>HHHHHHSSGLVPRGSHMQTTTVYSLEDLLPYLKQDNVDVKLAPGTYNVNGFDVGEDRLFSTTPLFLFEGSNSTYDFTDVKLNINTVVLTKFGNNEVNEIQILGNNNVLKNLKLEDIGTTAPSNRAQSIVIDGRDNRIEGFHLTIRGSYPYGYGDAFGKGGGSVINHRKHSGVLIRGLRNHLKDCTIISRSYGHIVAMQAASYPTVEGCYIEGEMRSTDDMLAEEGTGSPADKVDFMTVWGYKLPAGYMMSLQEGGIRAYNAGTTYIDGVEIQRATDNPTVLNCTIKNARTGVTLAHANGTKYVEGCTVLGCENGYSIGSGTVVNCGADAIYGPVFKNTYGSDKGYNADITILPPSDAYYNGHDAVAYIGGSNHNLTFRSEITEIPSNLKIMVSGDLQGLRVLHGSNPSQNNFAGTNIVLRNLTNFPVDLHSDSSNITVTSCDTDNITDNGTNNSIEAIDCDSD[2x]

FdlA from Flavobacterium sp. SA-0082 is an endo-type fucoidan-degrading enzyme that cleaves the sulfated fuco-glucuronomannan (SFGM) through a lytic mechanism. We show that the FdlA-NTD adopts a right-handed parallel β-helix fold, and possesses a substrate binding site composed of a long groove and a unique alkaline pocket. Our structural, biochemical, and enzymological analyses strongly suggest that FdlA-NTD utilizes catalytic residues different from other β-helix polysaccharide lyases, potentially representing a novel polysaccharide lyase family. Here, we report crystal structures and enzymological characterization of wild type (WT) and eight single mutants of the catalytic N-terminal domain (NTD) of FdlA, revealing its unique substrate binding pocket and identifying the key catalytic residues.

We first measured the enzymatic activity of 12 mutants and found that eight of them (D137A, K141A, H176A, F179A, E236A, R240A, Y242A, and Y242F) almost completely abolished their activities, H279A mutant retained approximately 65% of the activity compared with WT, while mutations of Asn243, Arg272, and Tyr322 to Ala only negligibly affect their activities. However, we identified changes around the potential active site in several inactive mutants, implying the potential roles of these residues in catalysis. Similar to R240A, the mutant form F179A also exhibited a structural rearrangement around the active site, with a 3.8 Å shift of the Tyr242 side chain towards Ala179. Therefore, mutation of Phe179 and His176 possibly results in the dysfunction of Tyr242 and hence loss of the catalytic activity of FdlA-NTD. As it constitutes the catalytic acid, the hydroxyl group of the Tyr242 side chain is essential for the enzymatic activity, and its improper positioning may severely affect the catalysis of the enzyme. Circular dichroism (CD) spectra showed that all inactive mutants possess similar secondary structures to the wild-type protein, indicating that the loss of activity of these mutants is due to the residue mutations, but not protein conformational changes.> YEQDKTYKITVLHTNDHH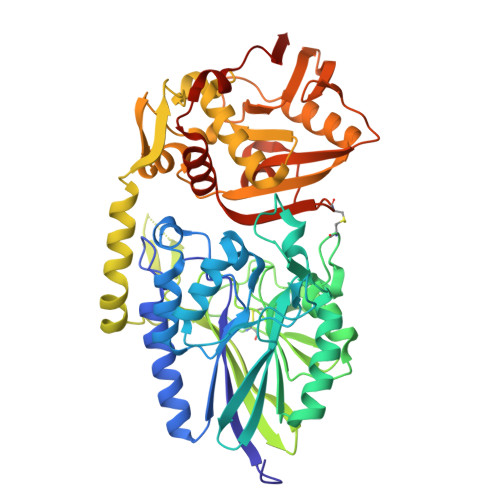GHFWRNEYGEYGLAAQKTLVDGIRKEVAAEGGSVLLLSGGDINTGVPESDLQDAEPDFRGMNLVGYDAMAIGNHEFDNPLTVLRQQEKWAKFPLLSANIYQKSTGERLFKPWALFKRQDLKIAVIGLTTDDTAKIGNPEYFTDIEFRKPADEAKLVIQELQQTEKPDIIIAATHMGHYDNGEHGCNAPGDVEMARALPAGSLAMIVGGHSQDPVCMAAENKKQVDYVPGTPCKPDQQNGIWIVQAHEWGKYVGRADFEFRNGEMKMVNYQLIPVNLKKKVTWEDGKSERVLYTPEIAENQQMISLLSPFQNKGKAQLEVKIGETNGRLEGDRDKVRFVQTNMGRLILAAQMDRTGADFAVMSGGGIRDSIEAGDISYKNVLKVQPFGNVVVYADMTGKEVIDYLTAVAQMKPDSGAYPQFANVSFVAKDGKLNDLKIKGEPVDPAKTYRMATLNFNATGGDGYPRLDNKCGYVNTGFIDAEVLKAYIQKSSPLDVSVYEPKGEVSWQEHHHHHH> SGRQISIRVQMLDDTQEVFEVSQRAPGKALFDLVCSHLNLVEGDYFGLEFQDQRKMIVWLDLLKPILKQIRRPKNIILRFVVKFFPPDHTQLLEELTRYLFALQIKHDLACGRLTC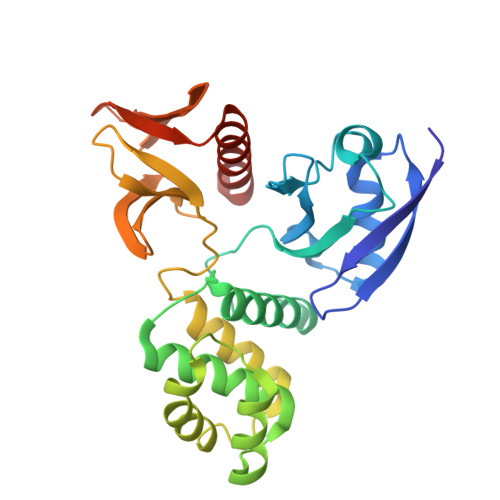NESSAALLVAHIVQSEIGDFDEVQCKQHLLNNKYIPEQDTLMDKIIGYHRKHVGQTPAESDYQLLEIARRLEMYGVRLHPAKDREGTRLSLAVAHSGVLVFQGHTKINAFNWSKVRKLSFKRKRFLIKLRPDLNSNCQDTLEFMMGSRDCCKVFWKICVEYHAFFRLFE> MWRSSGVSFTRYASEMAALLRQCLKEP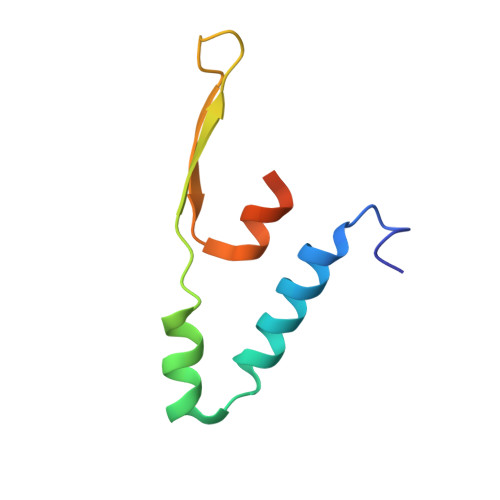YRTQAMQRNQIHLKETVYQQGQVLTRETFNDIKKAFEAAAKHAGEK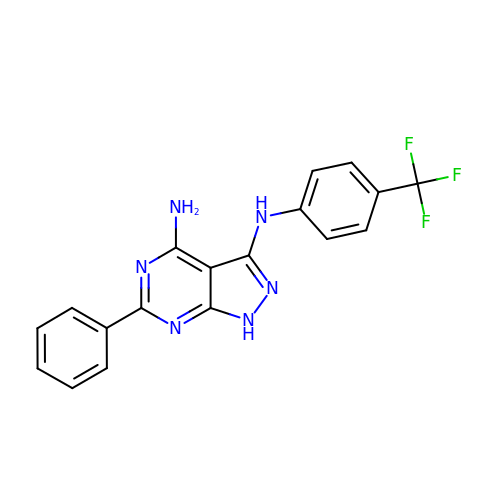6-phenyl-~{N}3-[4-(trifluoromethyl)phenyl]-1~{H}-pyrazolo[3,4-d]pyrimidine-3,4-diamine | C18 H13 F3 N6 | HYUDDHSPJFCULQ-UHFFFAOYSA-N>[2x]MKTVEIIEGIASGRTSARDVCEEALA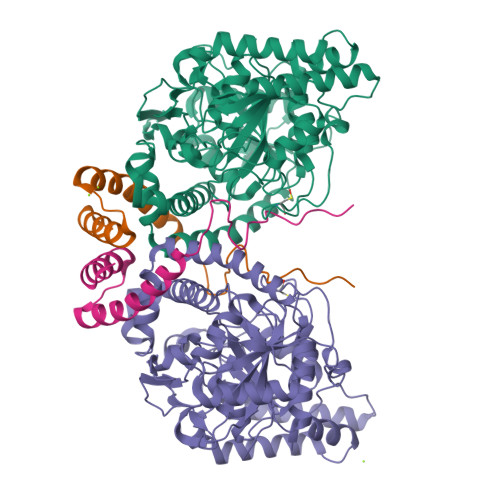TIGATDGLINAFTCRTVERARAEADAIDVRRARGEVLPPLAGLPYAVKNLFDIEGVTTLAGSKINRTLPPARADAVLVQRLKAAGAVLLGGLNMDEFAYGFTTENTHYGPTRNPHDTGRIAGGSSGGSGAAIAAGQVPLSLGSDTNGSIRVPASLCGVWGLKPTFGRLSRRGTYPFVHSIDHLGPLADSVEGLALAYDAMQGPDPLDPGCSASRIQPSVPVLSQGIAGLRIGVLGGWFRDNAGPAARAAVDVAALTLGASEVVMWPDAEIGRAAAFVITASEGGCLHLDDLRIRPQDFEPLSVDRFISGVLQPVAWYLRAQRFRRVYRDKVNALFRDWDILIAPATPISAPAIGTEWIEVNGTRHPCRPAMGLLTQPVSFAGCPVVAAPTWPGENDGMPIGVQLIAAPWNESLCLRAGKVLQDTGIARLKC;>MTETEIFAYIEAASIAIGIPLEPARARAVAHHFSRTALLAEMLESVPLSPESELAEIYRPAPFPAEDI[2x]(1S)-N-{(1S)-7,7-dihydroxy-1-[5-(2-methoxyquinolin-3-yl)-1H-imidazol-2-yl]nonyl}-6-ethyl-6-azaspiro[2.5]octane-1-carboxamide 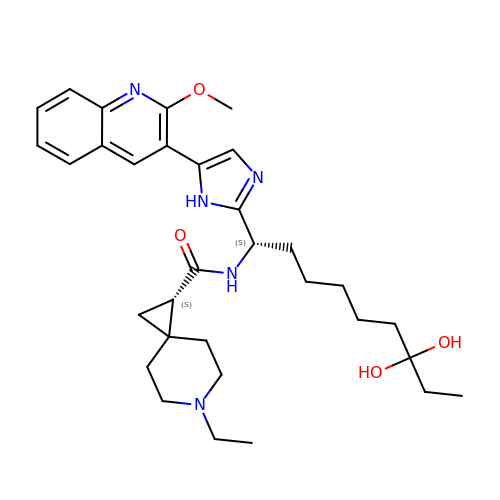| C32 H45 N5 O4 | YPIRISRXAGVBOC-RSXGOPAZSA-N>[2x]MVMLHSKNVKGFLENTLKPYDLHSVDFKTSSLQSSMIITATNG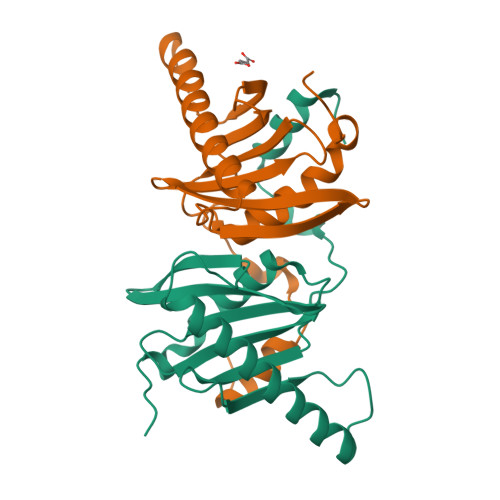GILSYATSNNDVPKNSINEINSVNNLKMMSLLIKDKWSEDENDTEEQHSNSCYPVEIDSFKTKIYTYEMEDLHTCVAQIPNSDLLLLFIAEGSFPYGLLVIKIERAMRELTDLFGYKLGLEHHHHHH>GSHMMGNKQTVFTHEQLEAYQDCTFFTRKEIMRLFYRYQDLAPQLVPLDYTTCPDVKVPYELIGSMPELKDNPFRQRIAQVFSEDGDGHMTLDNFLDMFSVMSEMAPRDLKAYYAFKIYDFNNDDYICAWDLEQTVTKLTRGELSAEE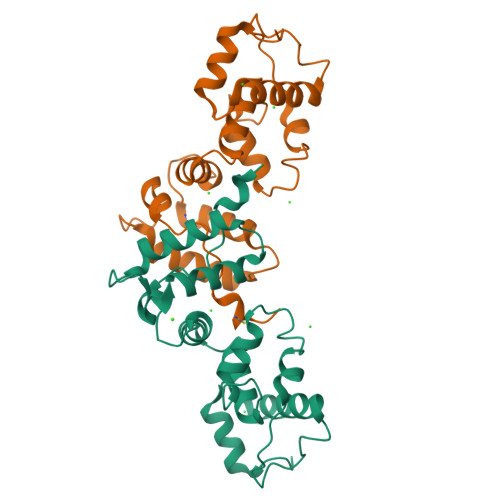VSLVCEKVLDEADGDHDGRLSLEDFQNMILRAPDFLSTFHIRI[2x]>AYVQGPPSPGYYPSSQITSLGFDQGYTNLWGPQHQRVDQGSLTIWLDSTSGSGFKSINRYRSGYFGANIK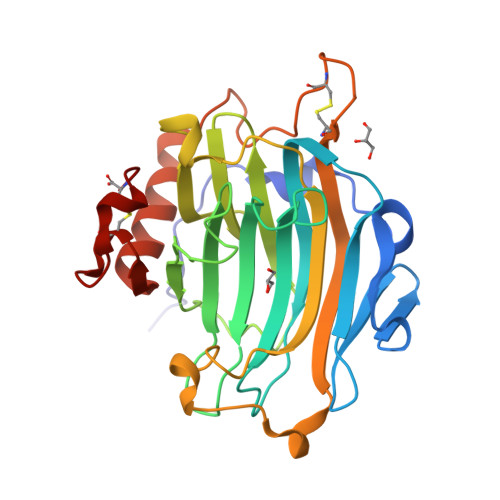LQSGYTAGVITSFYLSNNQDYPGKHDEIDIEFLGTIPGKPYTLQTNVFIEGSGDYNIIGREMRIHLWFDPTQDYHNYAIYWTPSEIIFFVDDVPIRRYPRKSDATFPLRPLWVYGSVWDASSWATENGKYKADYRYQPFVGKYEDFKLGSCTVEAASSCNPASVSPYGQLSQQQVAAMEWVQKNYMVYNYCDDPTRDHTLTPEC[3x]> MIPARFAGVLLALALILPGTLCAEGTRGRSSTARCSLFGSDFVNTFDGSMYSFAGYCSYLLAGGCQKRSFSIIGDFQNGKRVSLSVYLGEFFDIHLFVNGTVTQGDQRVSMPYASKGLYLETEAGYYKLSGEAYGFVARIDGSGNFQVLLSDRYFNKTCGLCGNFNIFAEDDFMTQEGTLTSDPYDFANSWALSSGEQWCERASPPSSSCNISSGEMQKGLWEQCQLLKSTSVFARCHPLVDPEPFVALCEKTLCECAGGLECACPALLEYARTCAQEGMVLYGWTDHSACSPVCPAGMEYRQCVSPCARTCQSLHINEMCQERCVDGCSCPEGQLLDEGLCVESTECPCVHSGKRYPPGTSLSRDCNTCICRNSQWICSNEECPGECLVTGQSHFKSFDNRYFTFSGICQYLLARDCQDHSFSIVIETVQCADDRDAVCTRSVTVRLPGLHNSLVKLKHGAGVAMDGQDVQLPLLKGDLRIQHTVTASVRLSYGEDLQMDWDGRGRLLVKLSPVYAGKTCGLCGNYNGNQGDDFLTPSGLAEPRVEDFGNAWKLHGDCQDLQKQHSDPCALNPRMTRFSEEACAVLTSPTFEACHRAVSPLPYLRNCRYDVCSCSDGRECLCGALASYAAACAGRGVRVAWREPGRCELNCPKGQVYLQCGTPCNLTCRSLSYPDEECNEACLEGCFCPPGLYMDERGDCVPKAQCPCYYDGEIFQPEDIFSDHHTMCYCEDGFMHCTMSGVPGSLLPDAVLSSPLSHRSKRSLSCRPPMVKLVCPADNLRAEGLECTKTCQNYDLECMSMGCVSGCLCPPGMVRHENRCVALERCPCFHQGKEYAPGETVKIGCNTCVCRDRKWNCTDHVCDATCSTIGMAHYLTFDGLKYLFPGECQYVLVQDYCGSNPGTFRILVGNKGCSHPSVKCKKRVTILVEGGEIELFDGEVNVKRPMKDETHFEVVESGRYIILLLGKALSVVWDRHLSISVVLKQTYQEKVCGLCGNFDGIQNNDLTSSNLQVEEDPVDFGNSWKVSSQCADTRKVPLDSSPATCHNNIMKQTMVDSSCRILTSDVFQDCNKLVDPEPYLDVCIYDTCSCESIGDCACFCDTIAAYAHVCAQHGKVVTWRTATLCPQSCEERNLRENGYECEWRYNSC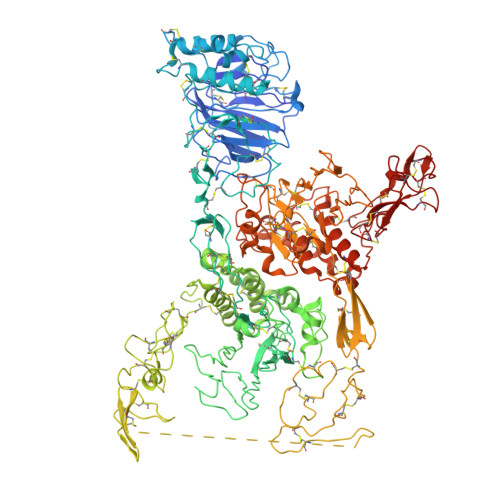APACQVTCQHPEPLACPVQCVEGCHAHCPPGKILDELLQTCVDPEDCP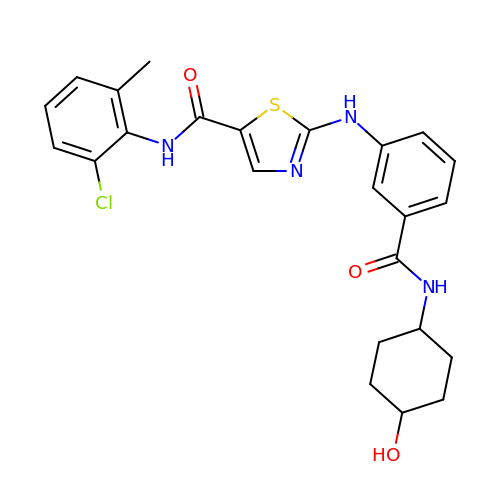~{N}-(2-chloranyl-6-methyl-phenyl)-2-[[3-[(4-oxidanylcyclohexyl)carbamoyl]phenyl]amino]-1,3-thiazole-5-carboxamide | C24 H25 Cl N4 O3 S | VWWJBXPDCCAIJW-SAABIXHNSA-N>[2x]SELRKLFYSADAVCFDVDSTVIREEGIDELAKICGVEDAVSEMTRRAMGGAVPFKAALTERLALIQPSREQVQRLIAEQPPHLTPGIRELVSRLQERNVQVFLISGG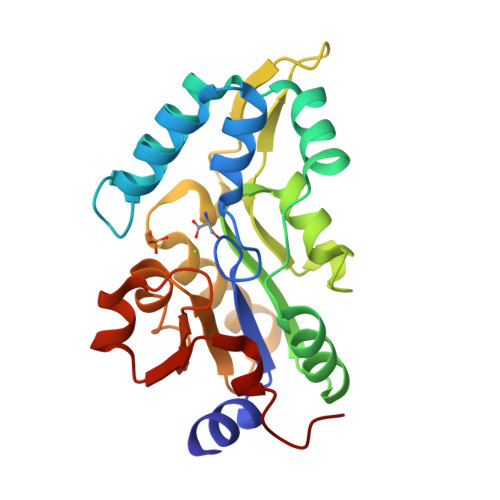FRSIVEHVASKLNIPATNVFANRLKFYFNGEYAGFDETQPTAESGGKGKVIKLLKEKFHFKKIIMIGDGATDMEACPPADAFIGFGGNVIRQQVKDNAKWYITDFVELLGELEE However, exceptionally high-level aminoglycoside-resistance is achieved by the action of intrinsic and acquired 16S ribosomal RNA (rRNA) methyltransferase enzymes in aminoglycoside-producing and human pathogenic bacteria, respectively. These resistance determinants block drug binding by catalyzing the transfer of a methyl group from their cosubstrate S-adenosyl-l-methionine (SAM) to the base of a defined target RNA nucleotide within the ribosomal A-site. Here, we describe detailed structural and functional analyses of one of these enzymes, the kanamycin-resistance methyltransferase from Catenulisporales acidiphilia (‘CacKam’). CacKam has a SAM-binding core fold comprised of a seven-stranded β-sheet with a central topological switch point, characteristic of Class I methyltransferases.

To assess the relative contributions of these two interactions to the observed β6/7 linker structure, individual D21A and W203A substitutions were created for further functional and structural analyses. CacKam-D21A had an activity equivalent to the wild-type enzyme as determined by the resistance conferred in E. coli to kanamycin (MIC >1024 μg/ml). Crystal structures were next determined for each CacKam variant to assess the effects of the D21A and W203A substitutions on β6/7 linker structure and crystal packing interaction. Despite the loss of a potentially important crystal packing contact, CacKam-D21A crystallized in the same space group as the wild-type enzyme with essentially identical unit cell parameters and crystal packing arrangement. Critically, the CacKam-D21A β6/7 linker adopts an identical extended conformation retaining the double cation-π stacking interaction of W203 with R43 and R73. Thus, only direct disruption of the interaction of W203 with R43/ R73 through the W203A substitution is sufficient to induce changes in the β6/7 linker structure and the crystal lattice. Together, these structures indicate that the R43/W203/R73 interaction is the major driver of the novel β6/7 linker structure observed in the crystal.

> MHHHHHHASGLVPRGSHMTRTTALKVLAGKKLTDLDPAEWAKAQASAERILVDVGTGDARTAYRQAIAHPEWLVVGVDPAWQRMTETAVRAARKPAKGGAPNLVLVSSAIETVPAALHGVADEVMVLMPWGKLLRGVVLGEADVLSGLRAVAKPGAPLEISIGTSIWREPIPLEIRDLPELTPETVVSTGLTDRLAALGWQVADVRLVPHTDLDTISSSWARRLGSGATETVLHLRAVAVDPRDPVGTQHPAAESAQDTPEEPQRDV> KHNRIKGIPKLDDANDAGGRNSTECTLILTEGDSAKTLAVSGLGVVGRDKYGVFPLRGKILNVREASHKQIMENAEINNIIKIVGLQYKKNYEDEDSLKTLRYGKIMIMTDQDQDGSHIKGLLINFIHHNWPSLLRHRFLEEFITPIVKVSKNKQEMAFYSLPEFEEWKSSTPNHKKWKVKYYKGLGTSTSKEAKEYFADMKRHRIQFKYSGPEDDAAISLAFSKKQ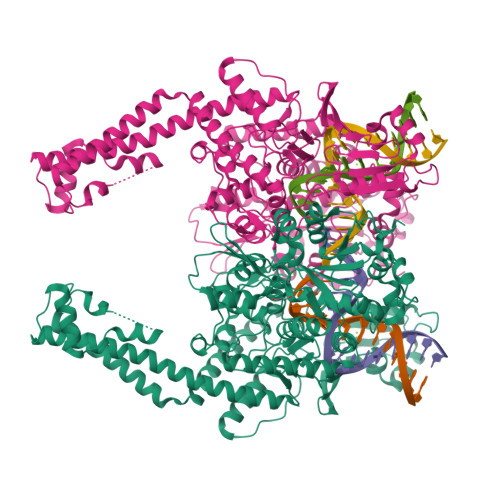IDDRKEWLTNFMEDRRQRKLLGLPEDYLYGQTTTYLTYNDFINKELILFSNSDNERSIPSMVDGLKPGQRKVLFTCFKRNDKREVKVAQLAGSVAEMSSYHHGEMSLMMTIINLAQNFVGSNNLNLLQPIGQFGTRLHGGKDSASPRYIFTMLSSLARLLFPPKDDHTLKFLYDDNQRVEPEWYIPIIPMVLINGAEGIGTGWSCKIPNFDVREIVNNIRRLMDGEEPLPMLPSYKNFKGTIEELAPNQYVISGEVAILNSTTIEISELPVRTWTQTYKEQVLEPMLNGTEKTPPLITDYREYHTDTTVKFVVKMTEEKLAEAERVGLHKVFKLQTSLTCNSMVLFDHVGCLKKYDTVLDILRDFFELRLKYYGLRKEWLLGMLGAESAKLNNQARFILEKIDGKIIIENKPKKELIKVLIQRGYDSDPVKAWKEAQQKVPDEEENEESDNEKETEKSDSVTDSGPTFNYLLDMPLWYLTKEKKDELCRLRNEKEQELDTLKRKSPSDLWKEDLATFIEELEAVEAKEKQDEQVGL>MLARKSIIPEEYVLARIAAENLRKPRIRDRLPKARFIAKSGACNLAHKNIREQGRFLQDIFTTLVDLKWRHTLVIFTMSFLCSWLLFAIMWWLVAFAHGDIYAYMEKGITEKSGLESAVCVTNVRSFTSAFLFSIEVQVTIGFGGRMMTEECPLAITVLILQNIVGLIINAVMLGCIFMKTAQAHRRAETLIFSRHAVIAVRNGKLCFMFRVGDLRKSMIISASVRIQVVKKTTTPEGEVVPIHQQDIPVDNPIESNNIFLVAPLIICHVIDKRSPLYDISATDLVNQDLEVIVILEGVVETTGITTQARTSYIAEEIQWGHRFVSIVTEEEGVYSVDYSKFGNTVRVAAPRCSARELDEKPSILIQTLQKSELSHQNSLRKRNSMRRNNSMRRSNSIRRNNSSLMVPKVQFMTPEGNQCPSES[4x];> MSLSFCGNNISSYNIYHGVLQNPCFVDALNLVPHVFLLFITFPILFIGWGSQSSKVQIHHNTWLHFPGHNLRWILTFALLFVHVCEIAEGIVSDSQRASRHLHLFMPAVMGFVATTTSIVYYHNIETSNFPKLLLALFLYWVMAFITKTIKLVKYWQLGWGMSDLRFCITGVMVILNGLLMAVEINVIRVRRYVFFMNPQKVKPPEDLQDLGVRFLQPFVNLLSKATYWWMNTLIISAHRKPIDLKAIGKLPIAMRAVTNYVCLKEAYEEQKKKAADHPNRTPSIWLAMYRAFGRPILLSSTFRYLADLLGFAGPLCISGIVQRVNEPKNNTTRFSETLSSKEFLENAHVLAVLLFLALILQRTFLQASYYVTIETGINLRGALLAMIYNKILRLSTSNLSMGEMTLGQINNLVAIETNQLMWFLFLCPNLWAMPVQIIMGVILLYNLLGSSALVGAAVIVLLAPIQYFIATKLAEAQKSTLDYSTERLKKTNEILKGIKLLKLYAWEHIFCKSVEETRMKELSSLKTFALYTSLSIFMNAAIPIAAVLATFVTHAYASGNNLKPAEAFASLSLFHILVTPLFLLSTVVRFAVKAIISVQKLNEFLLSDEIGEDSWRTGEGTLPFESCKKHTGVQSKPINRKQPGRYHLDNYEQARRLRPAETEDVAIKVTNGYFSWGSGLATLSNIDIRIPTGQLTMIVGQVGCGKSSLLLAILGEMQTLEGKVYWNNVNESEPSFEATRSRSRYSVAYAAQKPWLLNATVEENITFGSSFNRQRYKAVTDACSLQPDIDLLPFGDQTEIGERGINLSGGQRQRICVARALYQNTNIVFLDDPFSALDIHLSDHLMQEGILKFLQDDKRTVVLVTHKLQYLTHADWIIAMKDGSVLREGTLKDIQTKDVELYEHWKTLMNRQDQELEKDMEADQTTLERKTLRRAMYSREAKAQMEDEDEEEEEEEDEDDNMSTVMR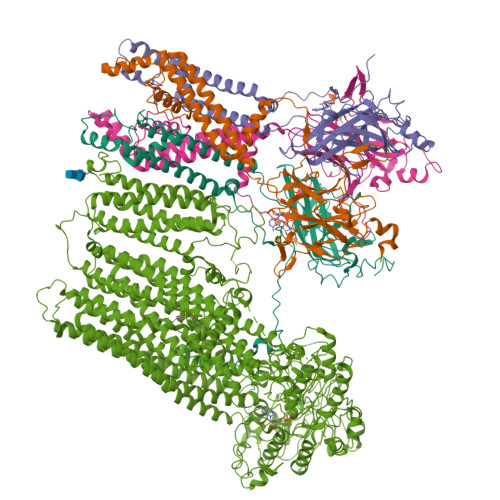LRTKMPWKTCWWYLTSGGFFLLFLMIFSKLLKHSVIVAIDYWLATWTSEYSINDPGKADQTFYVAGFSILCGAGIFLCLVTSLTVEWMGLTAAKNLHHNLLNKIILGPIRFFDTTPLGLILNRFSADTNIIDQHIPPTLESLTRSTLLCLSAIGMISYATPVFLIALAPLGVAFYFIQKYFRVASKDLQELDDSTQLPLLCHFSETAEGLTTIRAFRHETRFKQRMLELTDTNNIAYLFLSAANRWLEVRTDYLGACIVLTASIASISGSSNSGLVGLGLLYALTITNYLNWVVRNLADLEVQMGAVKKVNSFLTMESENYEGTMDPSQVPEHWPQEGEIKIHDLCVRYENNLKPVLKHVKAYIKPGQKVGICGRTGSGKSSLSLAFFRMVDIFDGKIVIDGIDISKLPLHTLRSRLSIILQDPILFSGSIRFNLDPECKCTDDRLWEALEIAQLKNMVKSLPGGLDATVTEGGENFSVGQRQLFCLARAFVRKSSILIMDEATASIDMATENILQKVVMTAFADRTVVTIAHRVHTILTADLVIVMKRGNILEYDTPESLLAQEDGVFASFVRADM> MERLWKDIKRDWLLYAMLLPTIIWFLIFLYKPMIGLQMAFKQYSAWKGIAGSPWIGFDHFVTLFQSEQFIRAIKNTLTLSGLSLLFGFPMPILLALMINEVYSKGYRKAVQTIVYLPHFISIVIVAGLVVTFLSPSTGVVNNMLSWIGLDRVYFLTQPEWFRPIYISSNIWKEAGFDSIVYLAAIMSINPALYESAQVDGATRWQMITRITLPCIVPTIAVLLVIRLGHILEVGFEYIILLYQPTTYETADVISTYIYRLGLQGARYDIATAAGIFNAVVALVIVLFANHMSRRITKTGVF;> MLATPFYSRSDRIFGIVNAVLLGIFALCALYPIIYIFSMSISSGAAVTQGRVFLLPVDIDFSAYGRVLHDKLFWTSYANTIFYTVFGVVTSLIFIVPGAYALSKPRIRGRRVFGFIIAFTMWFNAGMIPFFLNMRDLGLLDNRFGILIGFACNAFNIILMRNYFESISASFEEAARMDGANDLQILWKVYIPLAK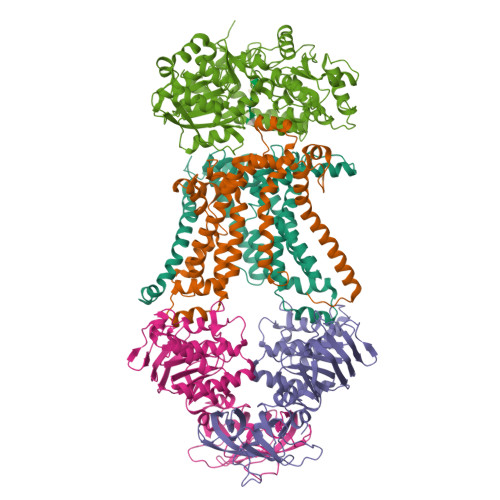PALATITLLCAISRWNGYFWAMVLLRAEEKIPLQVYLKKTIVDLNVNEEFAGALLTNSYSMETVVGAIIVMSIIPVIIVYPVVQKYFTKGVMLGGVKELEHHHHHHHHHH;> MKKMMLSVAAVATLMAFAAPVATAKEATWVTDKPLTLKIHMHFRDKWVWDENWPVAKESFRLTNVKLQSVANKAATNSQEQFNLMMASGDLPDVVGGDNLKDKFIQYGQEGAFVPLNKLIDQYAPHIKAFFKSHPEVERAIKAPDGNIYFIPYVPDGVVARGYFIREDWLKKLNLKPPQNIDELYTVLKAFKEKDPNGNGKADEVPFIDRHPDEVFRLVNFWGARSSGSDNYMDFYIDNGRVKHPWAETAFRDGMKHVAQWYKEGLIDKEIFTRKARAREQMFGGNLGGFTHDWFASTMTFNEGLAKTVPGFKLIPIAPPTNSKGQRWEEDSRQKVRPDGWAITVKNKNPVETIKFFDFYFSRPGRDISNFGVPGVTYDIKNGKAVFKDSVLKSPQPVNNQLYDMGAQIPIGFWQDYDYERQWTTPEAQAGIDMYVKGKYVMPGFEGVNMTREERAIYDKYWADVRTYMYEMGQAWVMGTKDVDKTWDEYQRQLKLRGLYQVLQMMQQAYDRQYKN;>[2x]MVASVSIQNVVKRYDKTTVVHGVSLDIEPGEFVVLVGPSGCGKSTTLRMVAGLEEISGGTIRIDGRVINDLAPKDRDVAMVFQNYALYPHLNVRDNISFGLRLKRTKKSVIDAAVKTAADILGLQPLLERKPSDLSGGQRQRVAMGRAIVRDPKVFLFDQPLSNLDAKLRTQMRAEIKRLHQRLGTTVIYVTHDQVEAMTLADRIVVMRDGLIEQIGKPMDLFLHPANTFVASFIGSPPMNLMPARIAVDSTQHVELNGGNRISLLPRAGTHLAPGQEVVFGIRPEDVTLDGVEGSERAQIKATVDIVEPLGSESILHATVGDHSLVVKVGGLNEVHPGDPVTLHVDLTRVHLFDAQSQASIY> GHMSRTVMCRKYHEELPGLDRPPYPGAKGEDI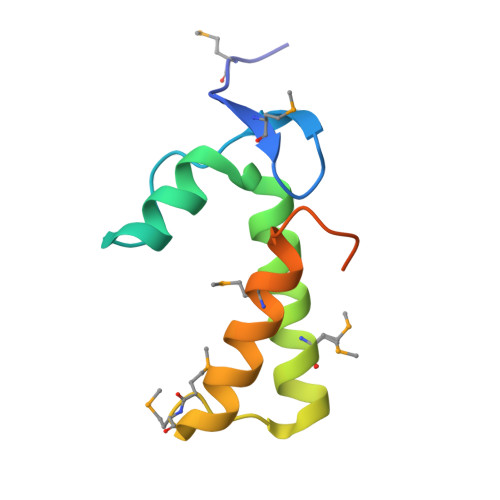YNNVSRKAWDEWQKHQTMLINERRLNMMNAEDRKFLQQEMDKFLSGEDYAKADGYVPPSAGS>[2x]GPLGSDLKDAEAVQKFFLEEIQLGEELLAQGDYEKG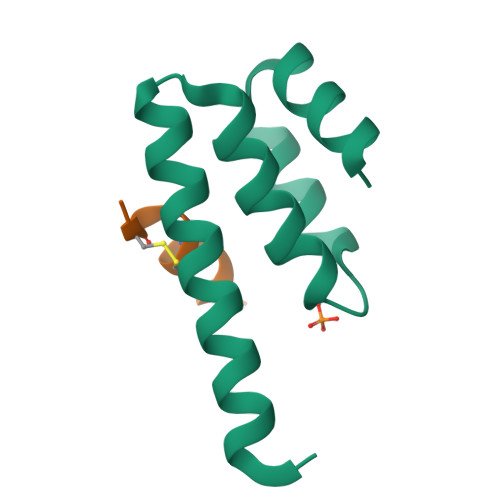VDHLTNAIAVCGQPQQLLQVLQQTLPPPVFQMLLTKL;>GCRLCRLLSYA[2x]3-[3-(4-chloranyl-3,5-dimethyl-phenoxy)propyl]-~{N}-(phenylsulfonyl)-1~{H}-indole-2-carboxamide | C26 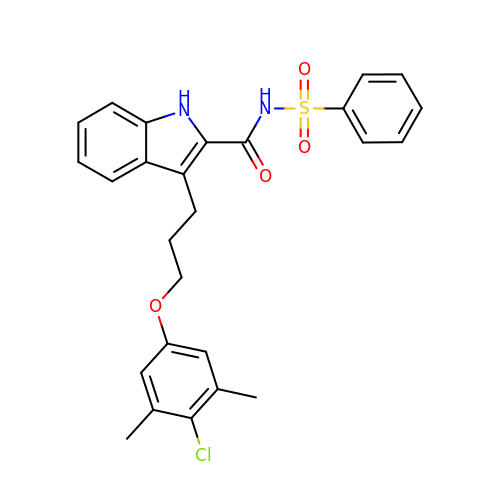H25 Cl N2 O4 S | SMGRUAFEHILHHU-UHFFFAOYSA-N>[2x]CUUGCUGAAG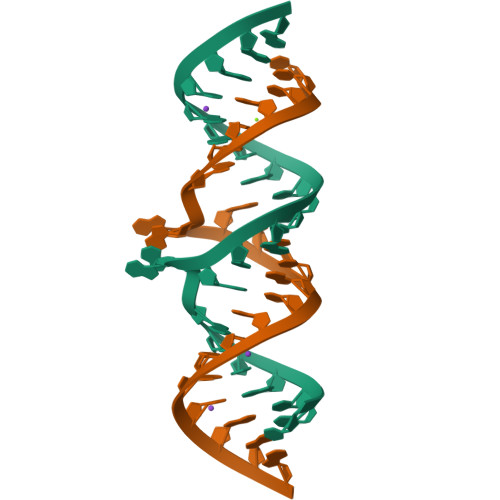CGCGCACGGCAAG2'-BROMO-4'-EPIDAUNORUBICIN | C27 H28 Br 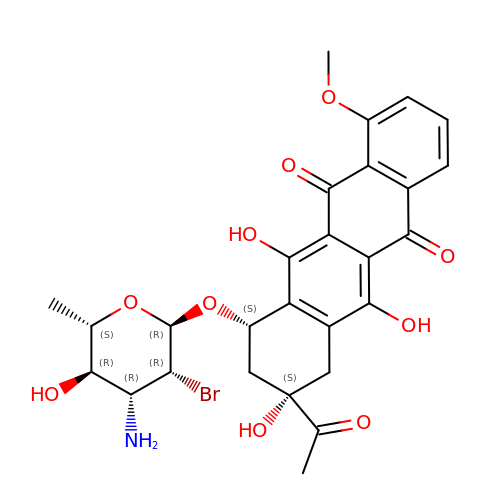N O10 | RNTSDANIDLGPLQ-VQBVCDDFSA-N>MTAQPNSLEARDIRYHLHSYTDAVRLEAEGPLVIERGDGIYVEDVSGKRYIEAMSGLWSVGVGFSEPRLAEAAARQMKKLPFYHTFSYRSHGPVIDLAEKLVSMAPVPMSKAYFTNSGSEANDTVVKLIWYRSNALGEPERKKIISRKRGYHGVTIASASLTGLPNNHRSFDLPIDRILHTGCPHFYREGQAGESEEQFATRLADELEQLIIAEGPHTIAAFIGEPVMGAGGVVVPPKTYWEKVQAVLKRYDILLIADEVICGFGRTGNLFGSQTFDMKPDILVMSKQLSSSYLPISAFLINERVYAPIAEESHKIGTLGTGFTASGHPVAAAVALENLAIIEERDLVANARDRGTYMQKRLRELQDHPLVGEVRGVGLIAGVELVTDKQAKTGLEPTGALGAKANAVLQ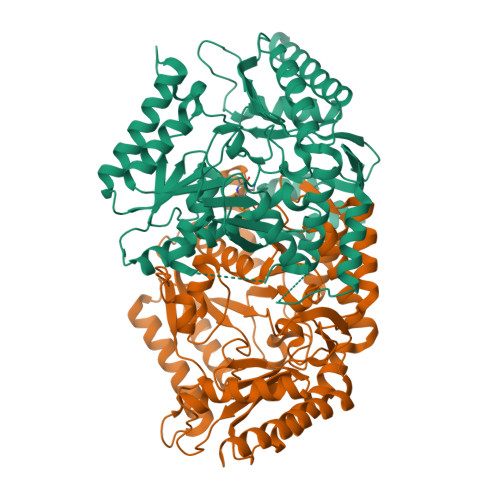ERGVISRAMGDTLAFCPPLIINDQQVDTMVSALEATLNDVQASLTR[2x]Enterovirus A71 (EV-A71) is the virus responsible for most of the severe forms of hand, foot and mouth disease (HFMD) associated with neurological involvement and mortality in young children under the age of 5. EV-A71 has been reported to bind to several cell surface receptors, including scavenger receptor B2 (SCARB2), P-selectin glycoprotein ligand-1 (PSGL1) and heparan sulfate (HS) glycosaminoglycan. Other host factors such as cyclophilin A, annexin II, sialylated glycans, vimentin, nucleolin, fibronectin and prohibitin have also been reported to promote infection, although their importance in viral entry is still less noted. It has been shown that EV-A71 interaction with PSGL1 on leukocytes requires the presence of sulfated tyrosine (Tyr) residues at the N-terminal region of PSGL1 and depends on two highly conserved lysine residues, VP1_244K and VP1_242K, near the 5-fold vertex of the viral capsid. Our data support a model of activity by which a single MADAL385 molecule binds on each of the 5-fold vertices of the EV-A71 capsid, thereby blocking the engagement of the virus with host receptors PSGL1 and/or HS.

To define the binding area of MADAL385 and to understand the possible mechanism underlying resistance and susceptibility to the compound, cryo-EM single particle analysis of MADAL385 bound to the EV-A71_11316 strain was performed. The corresponding three-dimensional (3D) maps were reconstructed at 3.3 and 3.6 Å resolutions, respectively, by applying icosahedral-symmetry averaging and using the images from a Falcon-3 direct electron detector. The atomic models of free and drug-bound EV-A71_11316 superimpose with an overall RMSD value of 0.292 Å, indicating that the incubation with MADAL did not cause any significant conformational change on the viral capsid proteins. In the two atomic models, the pocket factor lipid (sphingosine) has slightly different conformations, but the corresponding cryo-EM densities have similar intensities, suggesting that the drug binding likely induces subtle conformational changes around the pocket region but does not initiate pocket factor release. When the two 3D reconstructions were compared, strong extra densities were identified on the 5-fold vertices of the EV-A71_11316-MADAL385 complex, indicating that MADAL385 binds on the 5-fold vertex. The drug density fills the pore on the 5-fold symmetry axis and is connected to the capsid density. In particular, the intensity of MADAL385 density was highest at the symmetry axis, suggesting that the bound drug molecule occupies the very centric area of the 5-fold vertex. Due to steric hindrance and electrostatic repulsion, these observations suggest that only one molecule of MADAL385 binds on each vertex. Two other residues, VP1_244K and 245Y, with their corresponding side-chains extended towards MADAL385, are also found within the density envelope at the interface between capsid and drug.

> GDRVADVIESSIGDSVSRALTQALPAPTGQNTQVSSHRLDTGEVPALQAAEIGASSNTSDESMIETRCVLNSHSTAETTLDSFFSRAGLVGEIDLPLEGTTNPNGYANWDIDITGYAQMRRKVELFTYMRFDAEFTFVACTPTGQVVPQLLQYMFVPPGAPKPESRESLAWQTATNPSVFVKLTDPPAQVSVPFMSPASAYQWFYDGYPTFGEHKQEKDLEYGACPNNMMGTFSVRTVGSSKSKYPLVVRIYMRMKHVRAWIPRPMRNQNYLFKANPNYAGNSIKPTGTSRSAITTL;> SDRVAQLTIGNSTITTQEAANIIVGYGEWPSYCSDDDATAVDKPTRPDVSVNRFYTLDTKLWEKSSKGWYWKFPDVLTETGVFGQNAQFHYLYRSGFCIHVQCNASKFHQGALLVAILPEYVIGTVAGGTGTEDSHPPYKQTQPGADGFELQHPYVLDAGIPISQLTVCHHQRINLRTNNCATIIVPYMNTLPFDSALNHCNFGLLVVPISPLDFDQGATPVIPITITLAPMCSEFAGLRQAVTQ;> GFPTELKPGTNQFLTTDDGVSAPILPNFHPTPCIHIPGEVRNLLELCQVETILEVNNVPTNATSLMERLRFPVSAQAGKGELCAVFRADPGRDGPWQSTMLGQLCGYYTQWSGSLEVTFMFTGSFMATGKMLIAYTPPGGPLPKDRATAMLGTHVIWDFGLQSSVTLVIPWISNTHYRAHARDGVFDYYTTGLVSIWYQTNYVVPIGAPNTAYIIALAAAQKNFTMKLCKDTSHILQTASIQ;> MGSQVSTQRSGSHENSNSATEGSTINYTTINYYKDSYAATAGKQSLKQDPDKFANPVKDIFTEMAAPLKSPSAEACGY> SAQQYQGIYVWRVENFSHHLRNQEAGQPIVLHSPPFYTGRPGYKLCLRLHLQTPSAPRCSNFISLFVHTMQGEFDSQLSWPLQGTIRLAVLDQVEGQHHIEVMETKPDLQAFQRPTVMRNPKGFG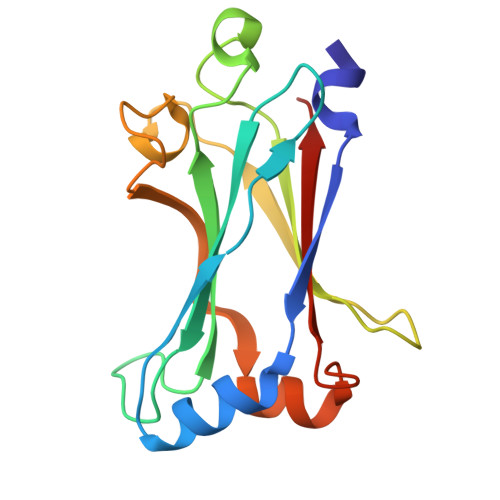YVTFLHLQALRQRGFVKEDVLLVRCEVTPRFD> MGSADASTFLNRVCGVSAARLTPCGTGTSTDVVYRAFDIYNEKVAGFAKFLKTNCCRFQEKDEEGNLLDSYFVVKRHTMSNYQHEETIYNLVKDCPAVAVHDFFKFRVDGDMVPHISRQRLTKYTMADLVYALRHFDEGNCDTLKEILVTYNCCDDDYFNKKDWYDFVENPDILRVYANLGERVRQSLLKTVQFCDAMRDAGIVGVLTLDNQDLNGNWYDFGDFVQVAPGCGVPIVDSYYSLLMPILTLTRALAAESHMDADLAKPLIKWDLLKYDFTEERLCLFDRYFKYWDQTYHPNCINCLDDRCILHCANFNVLFSTVFPPTSFGPLVRKIFVDGVPFVVSTGYHFRELGVVHNQDVNLHSSRLSFKELLVYAADPAMHAASGNLLLDKRTTCFSVAALTNNVAFQTVKPGNFNKDFYDFAVSKGFFKEGSSVELKHFFFAQDGNAAISDYDYYRYNLPTMCDIRQLLFVVEVVDKYFDCYDGGCINANQVIVNNLDKSAGFPFNKWGKARLYYDSMSYEDQDALFAYTKRNVIPTITQMNLKYAISAKNRARTVAGVSICSTMTNRQFHQKLLKSIAATRGATVVIGTSKFYGGWHNMLKTVYSDVETPHLMGWDYPKCDRAMPNMLRIMASLVLARKHNTCCNLSHRFYRLANECAQVLSEMVMCGGSLYVKPGGTSSGDATTAYANSVFNICQAVTANVNALLSTDGNKIADKYVRNLQHRLYECLYRNRDVDHEFVDEFYAYLRKHFSMMILSDDAVV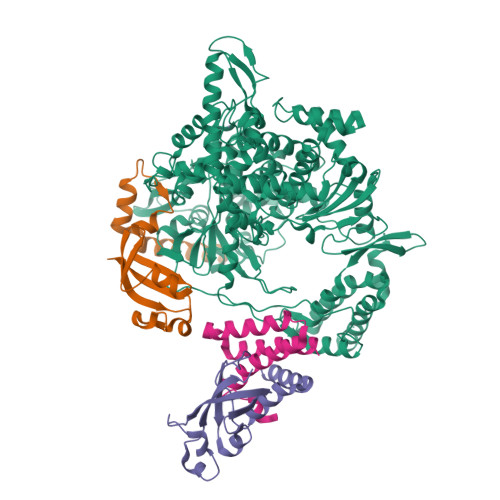CYNSNYAAQGLVASIKNFKAVLYYQNNVFMSEAKCWTETDLTKGPHEFCSQHTMLVKQGDDYVYLPYPDPSRILGAGCFVDDIVKTDGTLMIERFVSLAIDAYPLTKHPNQEYADVFHLYLQYIRKLHDELTGHMLDMYSVMLTNDNTSRYWEPEFYEAMYTPHTVLLVPRGSGHHHHHHAWSHPQFEK;>[2x]AIASEFSSLPSYAAYATAQEAYEQAVANGDSEVVLKKLKKSLNVAKSEFDRDAAMQRKLEKMADQAMTQMYKQARSEDKRAKVTSAMQTMLFTMLRKLDNDALNNIINNARDGCVPLNIIPLTTAAKLMVVVPDYGTYKNTCDGNTFTYASALWEIQQVVDADSKIVQLSEINMDNSPNLAWPLIVTALRANSAVKLQ;> GSKMSDVKCTSVVLLSVLQQLRVESSSKLWAQCVQLHNDILLAKDTTEAFEKMVSLLSVLLSMQGAVDINRLCEEMLDNRATLQ> MVMMTLYSGITCPFSHRCRFVLYEKGMDFEIKDIDIYNKPEDLAVMNPYNQVPVLVERDLVLHESNIINEYIDERFPHPQLMPGDPVMRGRGRLVLYRMEKELFNHVQVLENPAAANKEQAKAREAIGNGLTMLSPSFSKSKYILGEDFSMIDVALAPLLWRLDHYDVKLGKSAAPLLKYAERI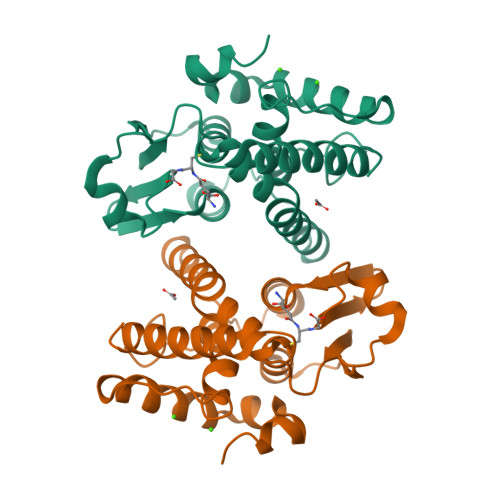FQREAFIEALTPAEKAMRKAENLYFQ> GSHMTKYKYTVEESERFNKHGIDLTVYGQVDPSATVVRVSVERGQFQEFFNVRSSYTYYVVSGQGVFYLNSEAVPAGATDLITVPPNTRIHYFGSMEMVLTVAPAFNEQDERHVRFISES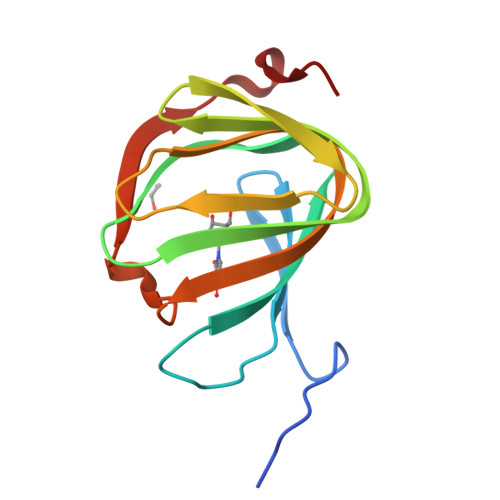ESPY>[2x]MNMFFRLTALAGLLAIAGQTFAVEDITRADQIPVLKEETQHATVSERVTSRFTRSHYRQFDLDQAFSAKIFDRYLNLLDYSHNVLLASDVEQFAKKKTELGDELRSGKLDVFYDLYNLAQKRRFERYQYALSVLEKPMDFTGNDTYNLDRSKAPWPKNEAELNALWDSKVKFDELSLKLTGKTDKEIRETLTRRYKFAIRRLAQTNSEDVFSLAMTAFAREIDPHTNYLSPRNTEQFNTEMSLSLEGIGAVYQMDDDYTVINSMVAGGPAAKSKAISVGDKIVGVGQTGKPMVDVIGWRLDDVVALIKGPKGSKVRLEILPAGKGTKTRTVTLTRERIRLEDRAVKMSVKTVGKEKVGVLDIPGFYVGLTDDVKVQLQKLEKQNVSSVIIDLRSNGGGALTEAVSLSGLFIPAGPIVQVRDNNGKVREDSDTDGQVFYKGPLVVLVDRFSAIASEIFAAAMQDYGRALVVGEPTFGKGTVQQYRSLNRIYDQMLRPEWPALGSVQYTIQKFYRVNGGSTQRKGVTPDIIMPTGNEETETGEKFEDNALPWDSIDAATYVKSGDLTAFEPELLKEHNARIAKDPEFQNIMKDIARFNAMKDKRNIVSLNYAVREKENNEDDATRLARLNERFKREGKPELKKLDDLPKDYQEPDPYLDETVNIALDLAKLEKARPAEQPAPVKHHHHHH

Prc (also named Tsp) is a member of the family of C-terminal processing proteases (CTPs) which features an embedded regulatory PDZ domain inserted into a serine protease domain. In Escherichia coli, Prc is involved in degrading abnormal proteins that are unfolded or partially folded and marked cotranslationally at the C terminus by an SsrA tag and that are exported to the periplasm through the Sec translocon. By associating with its adaptor protein, NlpI, Prc is also involved in the regulated proteolysis of MepS, a lipid-anchored hydrolase specific for PG cross-links. The activity of Prc strictly requires the PDZ domain, and the PDZ deletion completely abolishes the protease activity.

We determined the structure of Prc-S452I/L252Y, which is indeed trapped in the unliganded resting state. In the structure of Prc-S452I/L252Y, the PDZ domain is docked inside the bowl, interacting with residues, mainly from NHD and CHD, dispersed across a wide region; these residues constitute a total interface area of 1,595 Å2. Interestingly, the docked PDZ domain makes little contact with the protease domain; the only contact is made between the stacking side chains of PDZ Val278 and Phe449 at the back, and this contact anchors the PDZ domain in a specific position to expose the ligand-binding strand b4. Compared to the structure of the liganded activated state, in the structure of the unliganded resting state, the docked PDZ domain is repositioned to expose its ligand-binding site for the substrate C terminus to an open space above the platform. The two-β-stranded substrate-binding hinge, which is formed in the activated state and which connects the PDZ domain to helix h9 and the platform, is unfolded into two coils; the critical substrate-sensing residues Leu245 and Leu340 are separated and become solvent exposed. Helix h9 is drifted away and partially unfolded to make up the large vaulted space above the platform. Lastly, without a folded connecting hinge, the proteolytic platform is angled down with misaligned active-site residues: the catalytic Lys477 and Ser452 are apart from each other, and the amide groups of Ala453 and Gly398, forming the oxyanion pocket, are out of place. We found that limited V8 proteolysis indeed resulted in the two fragments from Prc-S452I/L252Y but not from Prc-K477A at various incubation times, supporting the flexibility of helix h9 in the resting state. For Prc-S452I/L252Y, crystals were obtained in a solution containing 0.2 M sodium thiocyanate (pH 6.4 to 6.8) and 20% PEG 3350. The crystals of Prc-S452I/L252Y were found to be merohedrally twinned with a twinning fraction of 0.42, as determined by the Phenix tool Xtriage and as subsequently checked by the CCP4 program TRUNCATE.> CUGGG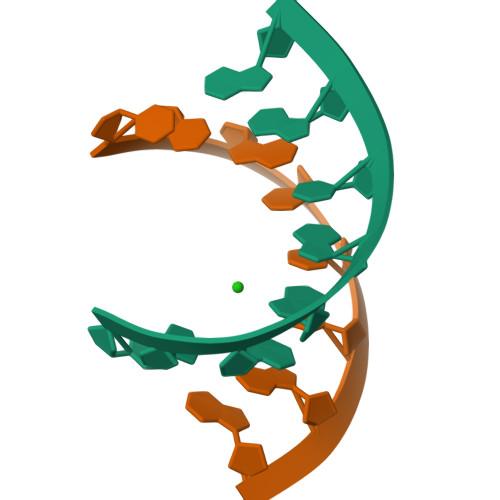CGG;> CCGCCUGG> APKAPADGLKMDKTKQPVVHNHSTHKAVKCGDCHHPVNGKEDYQKCATAGCHDNMDKKDKSAKGYYHAMHDKGTKF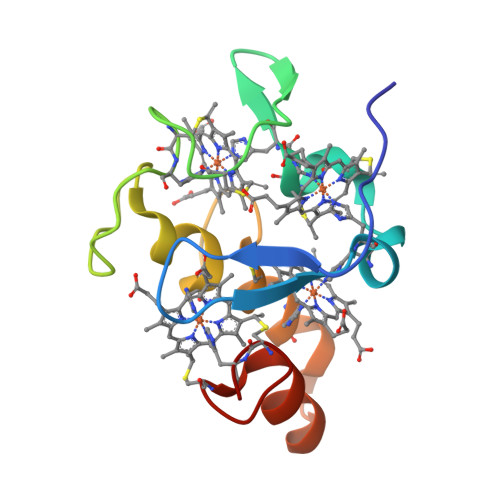KSCVGCHLETAGADAAKKKELTGCKGSKCHS> TPR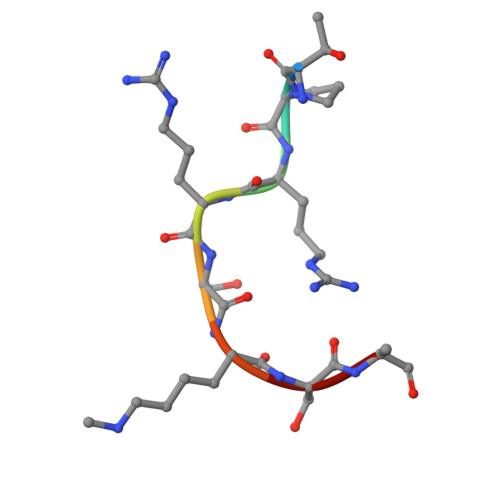RSKSA>[8x]MATTSNQNVEFVRTGYGKNMVKVLHIRREGNHHHIIELIANVQLTLKTRKDYLTGDNSDIIPTDTVKNTVHALAKLKGIKSIESFALDICEHFLTAFNHVTRVKVNIDEVPWKRLEKNGVEHNHAFIHCPEALRFCEAEQYLSKTPVVHSGLKDMKVLKTTQTGFEGFLRDRFTTLTDAKDRFFCTSVYARWRYNTINVAFDAAWKAVKDTVIQKFAGPYDRGEYSPSVQKTLYDTQLLVLDRIPEVEEIEIIMPNQHYFVIDMTKIGLSNKDEVYLPLDNPSGNITGTVCRKPRARM

Urate oxidase (uricase, Uox) catalyses hydroxylation of urate to give 5-hydroxyisourate (HIU). This is the first and rate-limiting step of uricolysis, a three-step enzymatic pathway present in both prokaryotes and eukaryotes that converts urate into the more soluble (S)-allantoin. The oldest known structure of the enzyme is a tetramer of the tunnelling (T) fold domain able to catalyse urate oxidation without the help of cofactors. The zebrafish (Danio rerio) urate oxidase (chr11: 8151055.8158017) encodes a protein of 298 aa with a C-terminal tripetide (ARM) corresponding to the type 1 peroxisome-targeting signal.

The crystal structure of DrUox was obtained at 2.8 Å resolution with a continuous electron density from Gly8 to Pro294. The DrUox structure shows the typical T-fold with a homotetramer organized as a dimer of dimers joining head-to-head to form the functional tetramer. Each monomer contains two tandem repeats of the T-fold domain forming an antiparallel β8-sheet with four main α-helices located at the concave side of the sheet. Two monomers assemble into a dimer by a two-fold axis to form a β16α8 barrel. The main dimerization interface is an antiparallel β-sheet formed by the N-terminal (aa 8–20) and C-terminal (aa 282–293) β strands of two subunits. The active sites (four in the tetramer) are located at the dimerization interfaces. In the crystal structure, chains A-C and B-D at the tetramer interface are connected by a disulfide bond involving Cys129, a residue not conserved in Uox sequences. The geometrical parameters of the disulfide, classify it as having a Left-Handed Staple conformation (+LHStaple), a rare bond characterized by a high strain energy. Phenylalanine 216, a residue strictly conserved in Uox alignment, is not part of the tetramer interface, but establishes main chain and side chain interaction with lysine 158 of the tetramer interface. F216 is not directly involved in substrate binding, but is involved in a cluster of hydrophobic interactions with active site residues.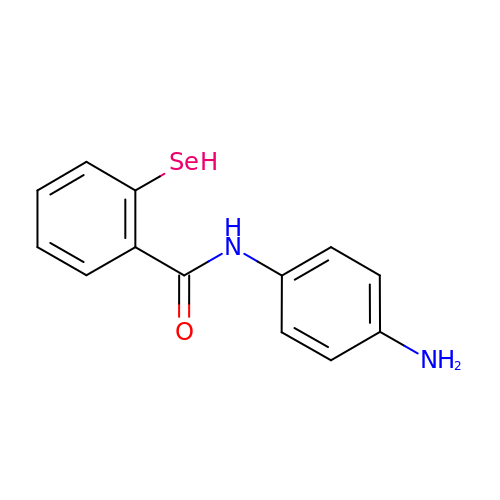~{N}-(4-aminophenyl)-2-selanyl-benzamide | C13 H12 N2 O Se | MAEAMJWLVXANNO-UHFFFAOYSA-N>[2x]MAHHHHHHSSGLEVLFQGPNTPVLEKNNVTLTGGGENVTKELKDKFTSGDFTVVIKYNQSSEKGLQALFGISNSKPGQQNSYVDVFLRDNGELGMEARDTSSNKNNLVSRPASVWGKYKQEAVTNTVAVVADSVKKTYSLYANGTKVVEKKVDNFLNIKDIKGIDYYMLGGVKRAGKTAFGFNGTLENIKFFNSALDEETVKKMTTNAVTGHLIYTANDTTGSNYFRIPVLYTFSNGRVFSSIDARYGGTHDFLNKINIATSYSDDNGKTWTKPKLTLAFDDFAPVPLEWPREVGGRDLQISGGATYIDSVIVEKKNKQVLMFADVMPAGVSFREATRKDSGYKQIDGNYYLKLRKQGDTDYNYTIRENGTVYDDRTNRPTEFSVDKNFGIKQNGNYLTVEQYSVSFENNKKTEYRNGTKVHMNIFYKDALFKVVPTNYIAYISSNDHGESWSAPTLLPPIMGLNRNAPYLGPGRGIIESSTGRILIPSYTGKESAFIYSDDNGASWKVKVVPLPSSWSAEAQFVELSPGVIQAYMRTNNGKIAYLTSKDAGTTWSAPEYLKFVSNPSYGTQLSIINYSQLIDGKKAVILSTPNSTNGRKHGQIWIGLINDDNTIDWRYHHDVDYSNYGYSYSTLTELPNHEIGLMFEKFDSWSRNELHMKNVVPYITFKIEDLKKN

S. pneumoniae produces up to three distinct sialidase enzymes: NanA, NanB, and NanC. NanC is an unusual sialidase in that its primary reaction product is 2-deoxy-2,3-didehydro-N-acetylneuraminic acid (Neu5Ac2en, also known as DANA), a nonspecific hydrolytic sialidase inhibitor. NanC adopts the same overall topology as seen in NanA and NanB, with a CBM (residues 85–271), followed by a catalytic domain (residues 272–740). The catalytic domain adopts the canonical glycoside hydrolase family 33 sialidase, six-bladed β-propeller fold shared by viral, bacterial, and mammalian sialidases.

The CBM presents a CBM family 40 (CBM40) β-sandwich fold with six-antiparallel strands forming a convex surface and five strands forming a concave, carbohydrate-binding side. Asp boxes, motifs typical of bacterial sialidases, are present in four of the β-propeller blades. Protruding from the catalytic domain is an I domain comprised mainly of β-strands (residues 403–498). The absent N-terminal residues include a signal sequence (residues 1–27) that was deleted to aid structural studies and a short region of unknown function (residues 28–84) of which electron density was only observed for residues 83 and 84. The binding site of the CBM is on the same side as the active site of the catalytic domain and the protein face on which they reside displays an overall positive charge. The NanC active site is a narrow constricted cleft, similar to NanB and contrary to NanA. A primary component of this constriction is the hydrophobic stack of Trp-716 and Tyr-632. These residues partially block the active site entrance providing specificity for α2–3-linked substrates as opposed to α2–6.6-(2,4-DIAMINO-6-ETHYLPYRIMIDIN-5-YL)-4-(3-METHOXYPROPYL)-2,2-DIMETHYL-2H-1,4-BENZOXAZIN-3(4H)-ONE | C20 H27 N5 O3 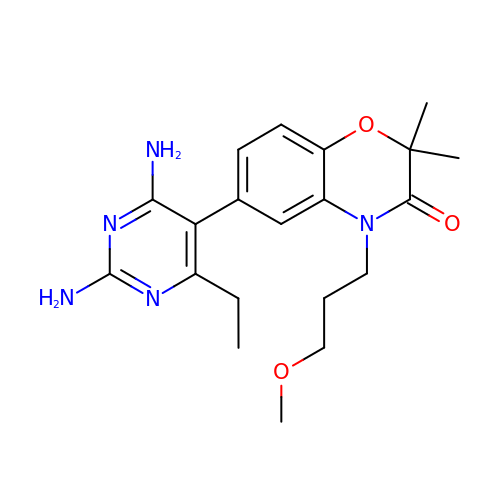| WPAPODFGOZXFLG-UHFFFAOYSA-N> MHSLLQYHISLYAPEQPSSLKSLLKPNERSADQLFIPNNIREDLTKKNLSILQVFPSSGKVIPSIVQDYFNLVPLNFNNNDFLNKTTLFKVFSNYDGKAYVLKRLPNIDKSMNPNKISKIYQIWSKINCTNLIKFRDIFQTTKFGNLSICLVFDYYPNSLSLYDYHFVNFPKFPITNNYLWIYLVQLTNVINSIHSQNLSIGNTLNWRKVLITGDP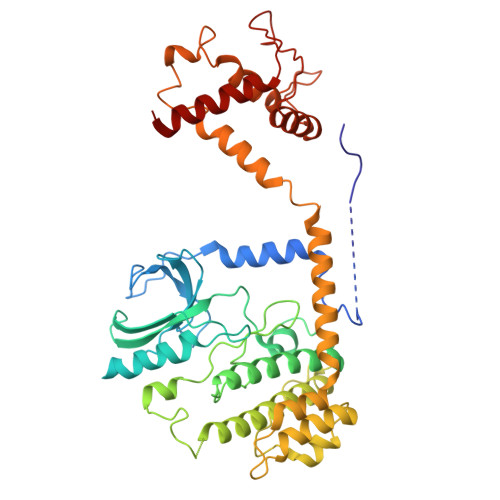GRIKLSHCNFMDLLFNDDTDTVVSSGGSTIEGQQQLDYKYLGELLFNLSINIENSNNNTAPKEYRLEEITPQSIDDMRQIDDKFKDVLKYLISDNGDSKKSIHDLTSHFYDKMFMVLESSQTYTEYMESVLSRELENGRLFRLVNKLNCIFGRIESRIDINWSESGTKFPIILFYDYVFHQVDSNGKPIMDLTHVLRCLNKLDAGIQEKLMLVTPDELNCIIISYKQLKDLIESTFRSITQA> KGGAXRH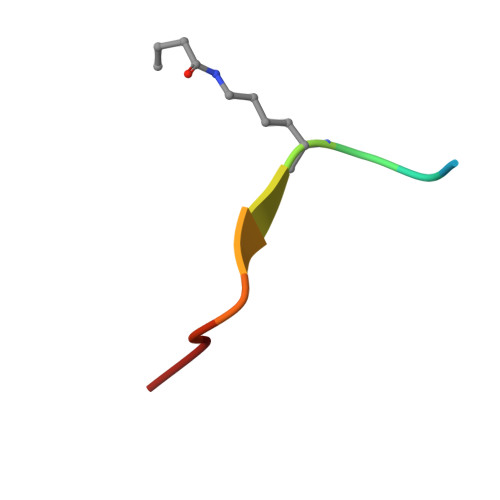RKIL> MSYKAQYTPGETQIAENRRKHMDPDYEFRKLREVSDEDLVKVLGHRNPGESYKSVHPPLDEMDFEEDIVRDMVEPIQGAKEGVRVRYIQFADSMYNAPAQPYDRARTYMWRYRGVDTGTLSGRQVIEMRELDLEGVSKELVETELFDPATTGIRGATVHGHSLRLDE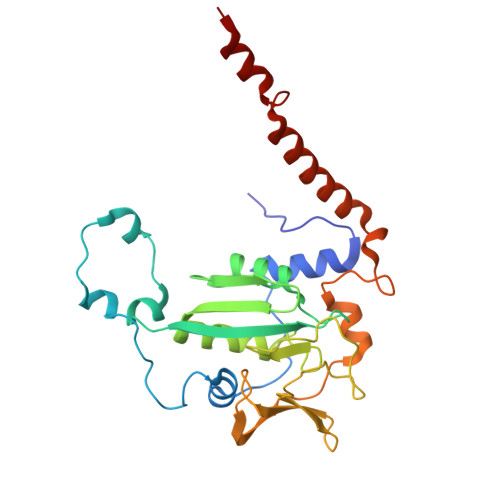NGLMFDALQRYVFDEEKGHVVYVKDQVGRPLDEPVDMGQPLGEDELKKITTIYRKDNIAMRDDKEAIEVVENIHTGRTLGGFGMDVFKDDLRKRLGDD ISG15 is a ubiquitin-like protein that is activated by an E1 enzyme (Uba7) and transferred to a cognate E2 enzyme (UBE2L6) to form a UBE2L6-ISG15 intermediate that functions with E3 ligases that catalyze conjugation of ISG15 to target proteins. E1 occupies the apex of the Ub/Ubl conjugation cascade where it performs two main functions: (1) specific activation of Ub/Ubl in a two-step process that results in the formation of a thioester bond between Ub/Ubl and an E1 catalytic cysteine (adenylation and thioester bond formation) and (2) recruitment of cognate E2 enzymes followed by transfer of Ub/Ubl to an E2 catalytic cysteine (thioester transfer). While Uba1 (E1) is specific to Ub activation, ISG15 is exclusively activated by Uba7 (E1) and specifically transferred to the E2 enzyme UBE2L6. Here, we present cryo-EM structures of human Uba7 in complex with UBE2L6, ISG15 adenylate, and ISG15 thioester intermediate in a conformational state that is poised for catalysis of Uba7-UBE2L6-ISG15 thioester transfer.

To gain insights into the molecular basis by which human Uba7 activates and transfers ISG15 to UBE2L6, we sought to determine the structure of a ‘doubly-loaded’ Uba7-UBE2L6-ISG15(t)/ISG15(a) mimetic complex. Previous studies in the Ub system have shown that although the single-loaded E1-E2-Ub(t) complex is capable of catalyzing thioester transfer, that double-loaded E1 is significantly more efficient at E2 recruitment and catalysis. To generate a mimetic of double-loaded Uba7-UBE2L6-ISG15(t)/ISG15(a) complex, free ISG15 and ATP/Mg2+ were mixed with purified singly-loaded Uba7-UBE2L6-ISG15(t) which allowed binding of ISG15 to the adenylation active site and adenylation of its C-terminal glycine, thus incorporating the ISG15 adenylate (ISG15(a)) into the complex. The double-loaded Uba7-UBE2L6-ISG15(t)/ISG15(a) complex was prepared and imaged by single-particle cryo-electron microscopy (cryo-EM). Two reconstructions of the Uba7-UBE2L6-ISG15(t)/ISG15(a) complex were subsequently isolated, which we refer to as Form 1 and Form 2, with overall nominal resolutions of 3.38 and 3.21 Å, respectively (masked at 0.143 FSC). Both reconstructions exhibit the same overall architecture and do not appear to be functionally different, with the main difference between them being the strength of ordering of the SCCH domain, ISG15(a) NTD, and ISG15(t) CTD. Globally, the Uba7-UBE2L6-ISG15(t)/ISG15(a) complex exhibits a conserved architecture in both forms of the complex with the AAD, IAD, and FCCH of Uba7 engaging ISG15(a) and UBE2L6 sandwiched between the UFD and SCCH of Uba7. Cryo-EM density linking Gly157 of the CTD of ISG15(t) to UBE2L6 L121K and linking UBE2L6 Cys86 and Uba7 Cys599 are clearly visible and only slight structural rearrangements would place the relevant atoms in position for catalysis, validating our strategy for trapping the complex.

> MDALDASKLLDEELYSRQLYVLGSPAMQRIQGARVLVSGLQGLGAEVAKNLVLMGVGSLTLHDPHPTCWSDLAAQFLLSEQDLERSRAEASQELLAQLNRAVQVVVHTGDITEDLLLDFQVVVLTAAKLEEQLKVGTLCHKHGVCFLAADTRGLVGQLFCDFGEDFTVQDPTEAEPLTAAIQHISQGSPGILTLRKGANTHYFRDGDLVTFSGIEGMVELNDCDPRSIHVREDGSLEIGDTTTFSRYLRGGAITEVKRPKTVRHKSLDTALLQPHVVAQSSQEVHHAHCLHQAFCALHKFQHLHGRPPQPWDPVDAETVVGLARDLEPLKRTEEEPLEEPLDEALVRTVALSSAGVLSPMVAMLGAVAAQEVLKAISRKFMPLDQWLYFDALDCLPEDGELLPSPEDCALRGSRYDGQIAVFGAGFQEKLRRQHYLLVGAGAIGCELLKVFALVGLGAGNSGGLTVVDMDHIERSNLSRQFLFRSQDVGRPKAEVAAAAARGLNPDLQVIPLTYPLDPTTEHIYGDNFFSRVDGVAAALDSFQARRYVAARCTHYLKPLLEAGTSGTWGSATVFMPHVTEAYRAPASAAASEDAPYPVCTVRYFPSTAEHTLQWARHEFEELFRLSAETINHHQQAHTSLADMDEPQTLTLLKPVLGVLRVRPQNWQDCVAWALGHWKLCFHYGIKQLLRHFPPNKVLEDGTPFWSGPKQCPQPLEFDTNQDTHLLYVLAAANLYAQMHGLPGSQDWTALRELLKLLPQPDPQQMAPIFASNLELASASAEFGPEQQKELNKALEVWSVGPPLKPLMFEKDDDSNFHVDFVVAAASLRCQNYGIPPVNRAQSKRIVGQIIPAIATTTAAVAGLLGLELYKVVSGPRPRSAFRHSYLHLAENYLIRYMPFAPAIQTFHHLKWTSWDRLKVPAGQPERTLESLLAHLQEQHGLRVRILLHGSALLYAAGWSPEKQAQHLPLRVTELVQQLTGQAPAPGQRVLVLELSCEGDDEDTAFPPLHYEL;>[2x]MGWDLTVKMLAGNEFQVSLSSSMSVSELKAQITQKIGVHAFQQRLAVHPSGVALQDRVPLASQGLGPGSTVLLVVDKCDEPLSILVRNNKGRSSTYEVRLTQTVAHLKQQVSGLEGVQDDLFWLTFEGKPLEDQLPLGEYGLKPLSTVFMNLRLRGG;> MASMRVVKELEDLQKKPPPYLRNLSSDDANVLVWHALLLPDQPPYHLKAFNLRISFPPEYPFKPPMIKFTTKIYHPNVDENGQICLPIISSENWKPSTKTSQVLEALNVLVNRPNIREPKRMDLADLLTQNPELFRKNAEEFTLRFGVDRPS>QAKHKQRKRLKSSCKRHPLYVDFSDVGWNDWIVAPPGYHAFYCHGECPFPLADHLNSTNHAIVQTLVNSVNSKIPKACCVPTELSAISMLYLDENEKVVLKNYQDMVVEGCGCR[2x];> QNLDSMLHGTGMKSDSDQKKSENGVTLAPEDTLPFLKCYCSGHCPDDAINNTCITNGHCFAIIEEDDQGETTLASGCMKYEGSDFQCKDSPKAQLRRTIECCRTNLCNQYLQPTLPPVVIGPFFDGSIR;> SGRGEAETRECIYYNANWELERTNQSGLERCEGEQDKRLHCYASWRNSSGTIELVKKGCWLDDFNCYDRQECVATEENPQVYFCCCEGNFCNERFTHL

Bone morphogenetic proteins (BMPs) and other members of the transforming growth factor-β (TGF-β) superfamily, like the activins, growth and differentiation factors (GDFs) and TGF-βs are secreted signaling proteins that regulate the development, maintenance and regeneration of tissues and organs. Members of the TGF-β superfamily bind two different types of serine/threonine-kinase receptors termed type I and type II receptors. In the present study we analyze the interaction of BMP-2 with its type I receptor BMPR-IA and its type II receptor ActR-IIB. ActR-II and ActR-IIB bind activin A (Act-A) with high affinity in the low nanomolar range leading to activation of the SMAD-2/-3 pathway, whereas binding of BMP-2 occurs with low-affinity in the micromolar range resulting in the activation of the SMAD-1/-5/-8 pathway.

The crystal structure of the ternary ligand-receptor complex of wildtype BMP-2 shows a dimeric ligand bound to only one BMPR-IAECD and ActR-IIBECD occupying the expected wrist (type I receptor binding site) and knuckle epitopes (type II receptor binding site). Both receptor ectodomains are located on the same half of the dimeric ligand, with the binding sites being almost identical to those identified in the crystal structures of the complexes BMP-2:BMPR-IA and BMP-7:ActR-II. The change in ligand-receptor stoichiometry in the crystal is clearly due to crystal packing as SDS-PAGE and RP-HPLC analyses proved this complex to be hexameric in solution. Inspection of the crystal lattice contacts shows that symmetry-related proteins block the empty epitopes. Inspection of the receptor-ligand interactions of both BMP-2/receptor complexes (comprising BMP-2 L100K/N102D, in the following termed ternary complex (1:2:2), or wildtype BMP-2, in the following termed ternary complex (1:1:1)) demonstrates that the ligand-receptor interfaces are highly similar. Superposition of the complexes yields an r.m.s. deviation of 0.3 Å for the Cα atoms of BMP-2 (in the ternary complex (1:1:1) only "bound" parts of BMP-2 were considered), and 0.4 Å for the Cα of BMP-2 and ActR-IIBECD. Analysis of the contact between ActR-IIBECD and wildtype BMP-2 indeed yields only five intermolecular polar bonds, one ion pair and four H-bonds. The H-bond between BMP-2 Ser88 Oγ and ActR-IIB Leu61 NH is in the center of the otherwise hydrophobic epitope, whereas the other polar bonds reside at the periphery. Comparing the affinities of the ActR-IIB variants L61P and L61A to wildtype BMP-2 shows no difference, indicating that, by contrast, in the wildtype environment the central H-bond does not contribute to the binding free energy. In the structure of the ternary complex (1:1:1) comprising wildtype BMP-2 the temperature factors of the equivalent residues Leu100 and Asn102 are higher than for nearby residues indicating increased flexibility.> MGHHHHHHGSMRRHAIILAAGKGTRMKSKKYKVLHEVAGKPMVEHVLESVKGSGVDQVVTIVGHGAESVKGHLGERSLYSFQEEQLGTAHAVQMAKSHLEDKEGTTIVVCGDTPLITKETLVTLIAHHEDANAQATVLSASIQQPYGYGRIVRNASGRLERIVEEKDATQAEKDINEISSGIFAFNNKTLFEKLTQVKNDNAQGEYYLPDVLSLILNDGGIVEVYRTNDVEEIMGVNDRVMLSQAEKAMQRRTNHYHMLNGVTIIDPDSTYIGPDVTIGSDTVIEPGVRINGRTEIGEDVVIGQYSEINNSTIENGACIQQSVVNDASVGANTKVGPFAQLRPGAQLGADVKVGNFVEIKKADLKDGAKVSHLSYIGDAVIGERTNIGCGTITVNYDGENKFKTIVGKDSFVGCNVNLVAPVTIGDDVLVAAGSTITDDVPNDSLAVARARQTTKEGYRK

One example is the bifunctional enzyme N‐acetylglucosamine 1‐phosphate uridyltransferase (GlmU) which completes one of the early cytoplasmic steps in the pathway, converting α‐D‐glucosamine 1‐phosphate (GlcN 1‐P) to uridine diphosphate‐N‐acetylglucosamine (UDP‐GlcNAc). This occurs in a two‐step process, with the acetyltransferase activity of GlmU first catalyzing the reaction of acetyl coenzyme A (AcCoA) and GlcN 1‐P to form CoA and N‐acetylglucosamine 1‐phosphate (GlcNAc 1‐P). Subsequently, the uridyltransferase activity of GlmU catalyzes the Mg2+‐dependent reaction of UTP with GlcNAc 1‐P to form UDP‐GlcNAc and pyrophosphate. We identified that Staphylococcus aureus GlmU (SaGlmU), which was previously targeted for inhibitor development, possesses a dual‐cysteine variation (C379/C404) within the acetyltransferase active site.

The overall fold was highly conserved in both structures, with an all‐atom RMSD of 0.76 Å. Both structures were obtained under reducing conditions in the presence of 0.5 mM DTT. The biological trimer assembly is captured in both structures and the oligomerization interface is largely comprised of the LβH of the acetyltransferase domain. Finally, the interface between the AcCoA and GlcN 1‐P sites of SaGlmU, where C379 and C404 are located, was compared to the corresponding region of SpGlmU. For the cocrystal structure of SaGlmU complexed with AcCoA and citrate, which was crystallized in the presence of DTT, this region closely resembled that of SpGlmU complexed with AcCoA. Position 379 differs between the two isozymes, with the additional thiol sidechain of C379 (SaGlmU) oriented away from the acetyl group. However, this does not introduce any notable structural differences compared to SpGlmU, with the sidechains of key catalytic residues E348 and H362 occupying the same positions in both enzymes (Sulzenbacher et al., 2001). C404 (SaGlmU) and S404 (SpGlmU) adopt the same orientation, both within hydrogen bonding distance to the thioester carbonyl of AcCoA, which is further stabilized by an additional hydrogen bond with the backbone amide of C379 (SaGlmU) or A379 (SpGlmU). Therefore, C404 is likely to share a similar role to S404 in the acetyltransferase reaction, which was proposed to facilitate recognition of AcCoA and/or stabilization of the resulting tetrahedral reaction intermediate (Sulzenbacher et al., 2001). Therefore, we propose that the acetyltransferase activity of SaGlmU is repressed under non‐reducing conditions due to disulfide formation between C379 and C404, which simultaneously clashes with AcCoA and prevents C404 from hydrogen bonding to the thioester carbonyl of AcCoA and the subsequent tetrahedral reaction intermediate.The Nef protein of human (HIV) and simian (SIV) immunodeficiency viruses is an important replication and pathogenicity factor. Nef-mediated internalization of CD4 from the surface of infected cells is highly conserved among primate lentiviruses and thought to promote the release of fully infectious viral particles and to prevent superinfection. Nef stimulates clathrin-mediated endocytosis of CD3, CD4 and other cellular receptors by acting as an adapter of the adapter protein machinery. Our study thus provides insights into the molecular basis for the versatility of Nef as an adapter protein for the internalization of surface molecules containing endocytic sorting motifs.

We were able to improve the crystal structure to 2.50 Å resolution by using an N-terminally truncated SIVmac239 Nef starting at M87 before the extended acidic cluster in SIV Nef. As before, a synthetic peptide of 16 residues comprising the cytoplasmic dileucine motif of CD4 was added to the crystallization screens. Again, the sorting motif of one Nef molecule in the asymmetric units contacts the hydrophobic crevice of another Nef molecule. In this structure, the electron density map was visible for all residues in the dileucine-based sorting motif, providing detailed molecular insights into the interaction of Nef with endocytic sorting motifs. Additional density of a helical conformation is visible in a solvent channel between both Nef subunits. This sequence could not be unambiguously assigned as only the main chain of two helical turns is defined. Upon binding to the hydrophobic crevice, the ExxxLM sorting motif of SIVmac239 Nef forms a regular α-helix (αL) of two turns ranging from E188 to M195, thereby ending with the last canonical residue of the internalization motif. The negatively charged hydroxyl side chain group of E190 aligns between the two positively charged guanidinium ion groups of arginines 137 and 138, forming two strong salt bridges in the assembly between the sorting motif and its recognition domain. L194 binds central to the hydrophobic crevice with contacts formed to G128, L129, I132 and R138 of Nef. Of note, no water molecules were seen in the binding interface between Nef and the sorting motif, indicating that the side chains of L194 and M195 sufficiently fill the hydrophobic crevice.

>[2x]GAMDDIDEEDDDLVGVSVRPKVPLRTMSYKLAIDMSHFIKEKGGLEGIYYSARRHRILDIYLEKEEGIIPDWQDYTSGPGIRYPKTFGWLWKLVPVNVSDEAQEDEEHYLMHPAQTSQWDDPWGEVLAWKFDPTLAYTYEAYVRYPEEFGS>[5x]GKAVHVIPRPHTDVEKILGGSGGSEALGMVETKGLTAAIEAADAMVASANVMLV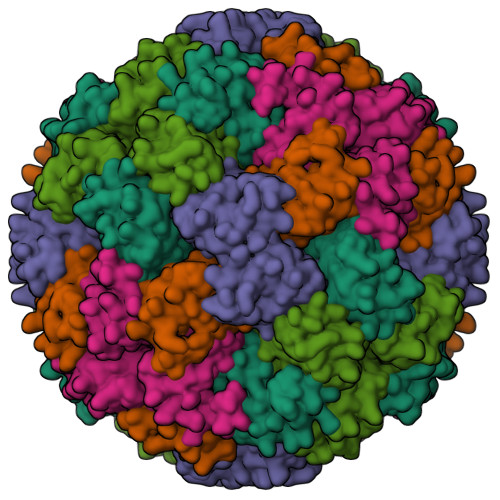GYEKIGSGLVTVIVRGDVGAVKAATDAGAAAARNVG> TELTLKPGTLTLAQLRAIHAAPVRLQLDASAAPAIDASVACVEQIIAEDRTAYGINTGFGLLASTRIASHDLENLQRSLVLSHAAGIGAPLDDDLVRLIMVLKINSLSRGFSGIRRKVIDALIALVNAEVYPHIPLKGSVGASGDLAPLAHMSLVLLGEGKARYKGQWLSATEALAVAGLEPLTLAAKEGLALLNGTQASTAYALRGLFYAEDLYAAAIACGGLSVEAVLGSRSPFDARIHEARGQRGQIDTAACFRDLLGDSSEVSLSHKNADKVQDPYSLRCQPQVMGACLTQLRQAAEVLGIEANAVSDNPLVFAAEGDVISGGNFHAEPVAMAADNLALAIAEIGSLSERRISLMMDKHMS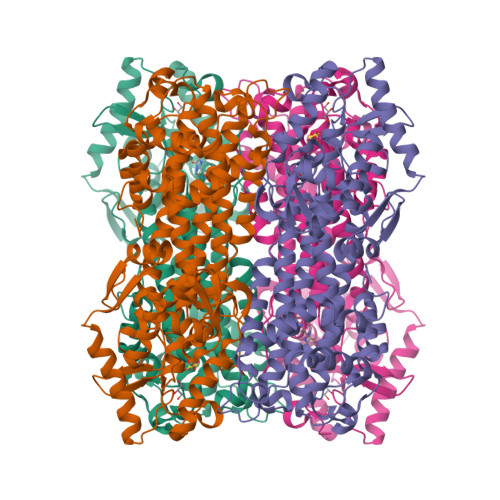QLPPFLVENGGVNSGFMIAQVTAAALASENKALSHPHSVDSLPTSANQEDHVSMAPAAGKRLWEMAENTRGVLAIEWLGACQGLDLRKGLKTSAKLEKARQALRSEVAHYDRDRFFAPDIEKAVELLAKGSLTGLLPAGVLPSL> GAMGSVNIPRKEKDFQGMLEYKKEDEQKLVKNLILELKPRGVAVNLIPGLPAYILFMCVRHADYLNDDQKVRSLLTSTINSIKKVLKKRGDDFETVSFWLSNTCRFLHC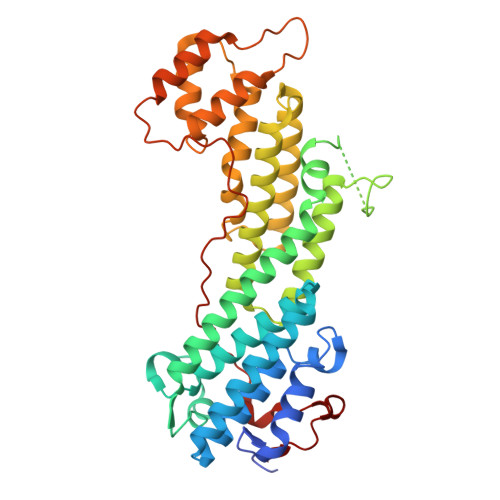LKQYSGEEGFMKHNTSRQNEHCLTNFDLAEYRQVLSDLAIQIYQQLVRVLENILQPMIVSGMLEHETIQGVSGVKPTGLRKRTSSIADEGTYTLDSILRQLNSFHSVMCQHGMDPELIKQVVKQMFYIIGAITLNNLLLRKDMCSWSKGMQIRYNVSQLEEWLRDKNLMNSGAKETLEPLIQAAQLLQVKKKTDDDAEAICSMCNALTTAQIVKVLNLYTPVNEFEERVSVSFIRTIQMRLRDRKDSPQLLMDAKHIFPVTFPFNPSSLALETIQIPASLGLGFISRV> GSHMPNFSGNWKIIRSENFEELLKVLGVNVMLRKIAVAAASKYAVEIKQEGDTFYIKVSTTVYT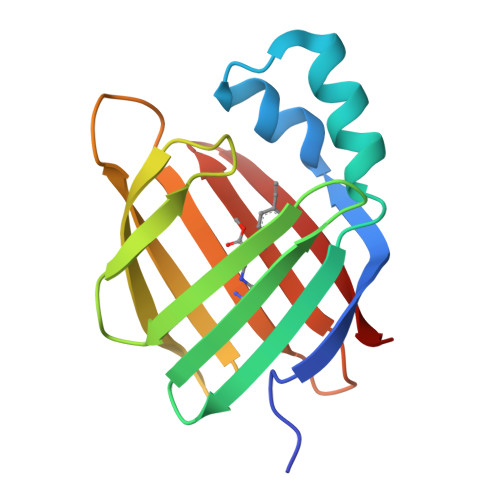TEINFKVGEEFEEQTVDGRPCKSLVKWESENKMVCEQKLLKGEGPKTSWTKELTNDGELILTMTADDVVCTQVFVRE paromamine 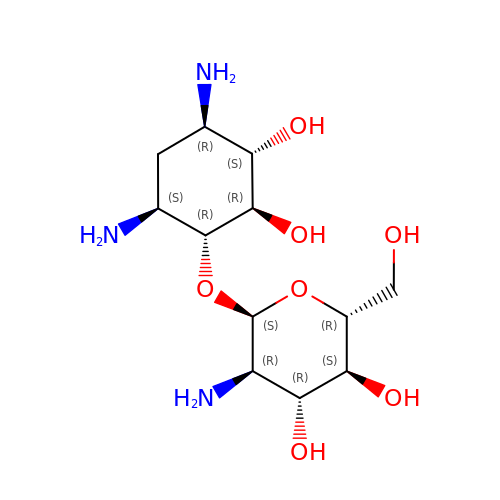| C12 H25 N3 O7 | JGSMDVGTXBPWIM-HKEUSBCWSA-N>[4x]AMKKDSKAPCVEVFDERDGCKAAGTQKASGDDGFCVKVS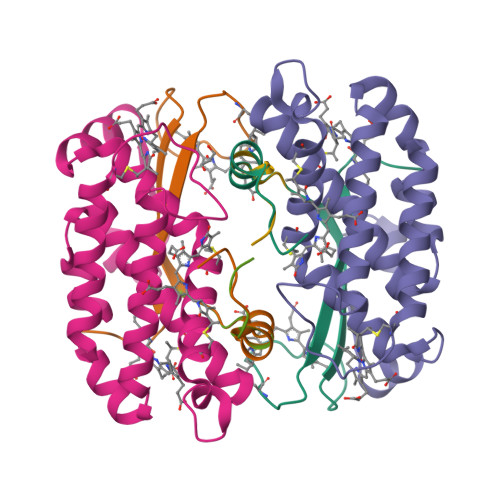MKAIGFNAAEAASVTKNYGIKRFGAKSV;>[4x]MLDAFSKVITSADGKAAYVGGADLQALKKFVSEGNKRMDSVNAIVSNASCIVSDSVSGMVCENPSLIAPNGGVYTNRKMAACLRDAEIILRYVSYSLLSGDSSVLEDRCLNGLKETYASLGVPAAGNARTISIMKATVIGFITNNSQQKKLSTPAGDCSALASEVGGYFDKVSSALA;>AMKKDSKAPCVEVFDERDGCKAAGTQKASGDDGFCVKVSMKAIKMNAAEATSVTKNYNTKLL[4x]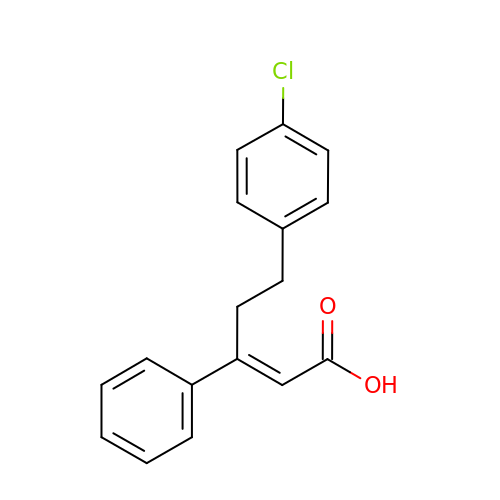(2Z)-5-(4-chlorophenyl)-3-phenylpent-2-enoic acid | C17 H15 Cl O2 | LLJYFDRQFPQGNY-QINSGFPZSA-N(2-MERCAPTOMETHYL-4-PHENYL-BUTYRYLIMINO)-(5-TETRAZOL-1-YLMETHYL-THIOPHEN-2-YL)-ACETIC ACID 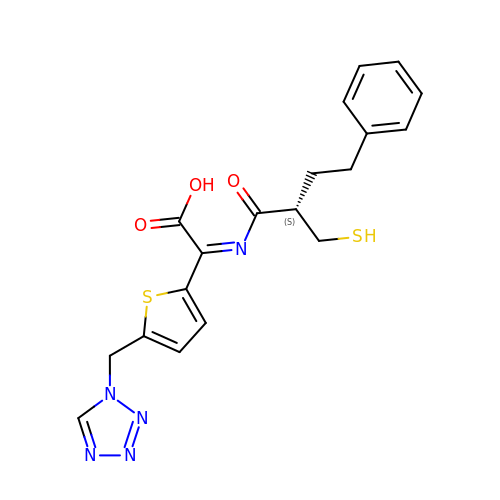| C19 H19 N5 O3 S2 | DUKDFMPUZRDWLT-CQSZACIVSA-N> DYKDDDDAMEPSATPGAQMGVPPGSREPSPVPPDYEDEFLRYLWRDYLYPKQYEWVLIAAYVAVFVVALVGNTLVCLAVWRNHHMRTVTNYFIVNLSLADVLVTAICLPASLLVDITESWLFGHALCKVIPYLQAVSVSVKVLTLSFIALDRWYAICHPLLFKSTARRARGSILGIWAVSLAIMVPQAAVMECSSVLPELANRTRLFSVCDERWADDLYPKIYHSCFFIVTYLAPLGLMAMAYFQIFRKLWGRQGIDCSFWNESYLTGSRDERKKSLLSKFGMDEGVTFMFIGRFDRGQKGVDVLLKAIEILSSKKEFQEMRFIIIGKGDPELEGWARSLEEKHGNVKVITEMLSREFVRELYGSVDFVIIPSYFEPFGLVALEAMCLGAIPIASAVGGLRDIITNETGIL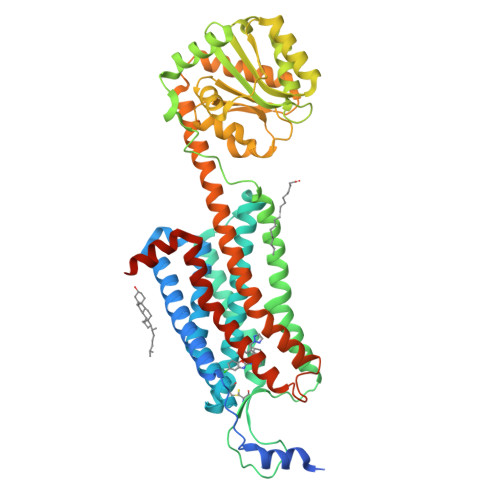VKAGDPGELANAILKALELSRSDLSKFRENCKKRAMSFSKQMRARRKTAKMLMVVLLVFALCYLPISVLNILKRVFGMFRQASDREAVYACFTFSHWLVYANSAANPIIYNFLSGKFREQFKAAFSCCLPGLHHHHHHHHHH>GPGSMVVAVDGPSGTGKSSVAKELARQLGASYLDTGAMYRIVTLWVLRAGVDLTDPAAIAAATDQVPMSVSSDPDAQTALLAGEDVSVPIRGNEVTGAVSAVSAVPAVRERLVRQQRELAESSGAVVVEGRDIGTVVLPDADVK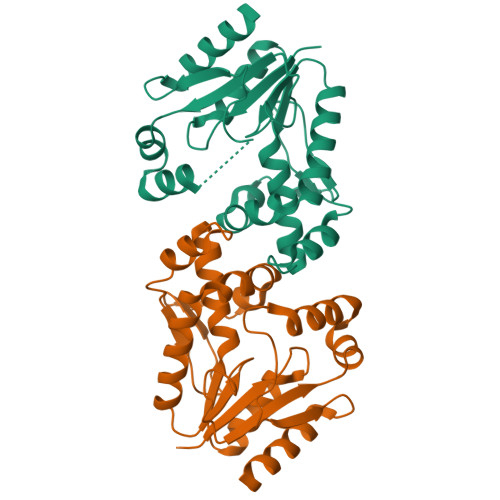IYLTASAQARAQRRNAQNVSGGGDDEYEKVLADVQRRDHLDSTRAVSPLRPAEDALEVDTSDMTQEQVVAHLLDLVRTRAGASR[2x]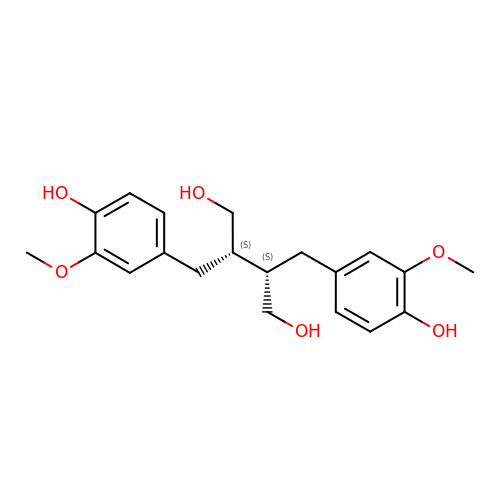(2S,3S)-2,3-bis[(3-methoxy-4-oxidanyl-phenyl)methyl]butane-1,4-diol | C20 H26 O6 | PUETUDUXMCLALY-HZPDHXFCSA-N> MEYWHYVET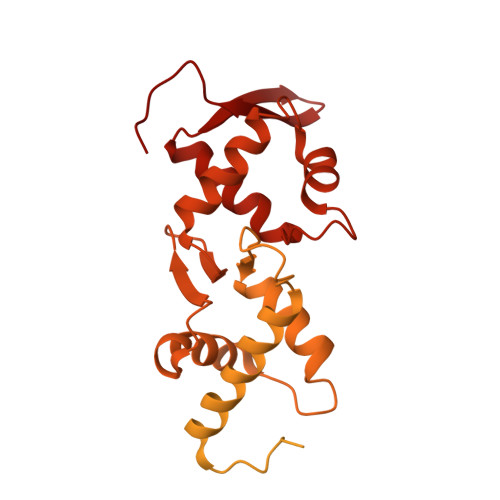TSSGQPLLREGEKDIFIDQSVGLYHGKSKILQRQRGRIFLTSQRIIYIDDAKPTQNSLGLELDDLAYVNYSSGFLTRSPRLILFFKDPSSKDELGKSAETASADVVSTWVCPICMVSNETQGEFTKDTLPTPICINCGVPADYELTKSSINCSNAIDPNANPQNQFGVNSENICPACTFANHPQIGNCEICGHRLPNASKVRSKLNRLNFHDSRVHIELEKNSLARNKSSHSALSSSSSTGSSTEFVQLSFRKSDGVLFSQATERALENILTEKNKHIFNQNVVSVNGVDMRKGASSHEYNNEVPFIETKLSRIGISSLEKSRENQLLNNDILFNNALTDLNKLMSLATSIERLYKNSNITMKTKTLNLQDESTVNEPKTRRPLLILDREKFLNKELFLDEIAREIYEFTLSEFKDLNSDTNYMIITLVDLYAMYNKSMRIGTGLISPMEMREACERFEHLGLNELKLVKVNKRILCVTSEKFDVVKEKLVDLIGDNPGSDLLRLTQILSSNNSKSNWTLGILMEVLQNCVDEGDLLIDKQLSGIYYYKNSYWPSHI However, exceptionally high-level aminoglycoside-resistance is achieved by the action of intrinsic and acquired 16S ribosomal RNA (rRNA) methyltransferase enzymes in aminoglycoside-producing and human pathogenic bacteria, respectively. These resistance determinants block drug binding by catalyzing the transfer of a methyl group from their cosubstrate S-adenosyl-l-methionine (SAM) to the base of a defined target RNA nucleotide within the ribosomal A-site. Here, we describe detailed structural and functional analyses of one of these enzymes, the kanamycin-resistance methyltransferase from Catenulisporales acidiphilia (‘CacKam’). CacKam has a SAM-binding core fold comprised of a seven-stranded β-sheet with a central topological switch point, characteristic of Class I methyltransferases.

To assess the relative contributions of these two interactions to the observed β6/7 linker structure, individual D21A and W203A substitutions were created for further functional and structural analyses. In contrast, substitution of the universally conserved W203 to alanine resulted in complete loss of resistance, consistent with previous analyses of equivalent substitutions in KamB and NpmA. In contrast, although CacKam-W203A also crystallized in space group P212121, the substitution results in a new unit cell with an altered packing arrangement and two molecules in the asymmetric unit. Changes in the CacKam-W203A structure are confined to the β6/7 linker, which is disordered in both chains. Additionally, D21 is no longer involved in crystal packing interactions made by either CacKam-W203A molecule. Thus, only direct disruption of the interaction of W203 with R43/ R73 through the W203A substitution is sufficient to induce changes in the β6/7 linker structure and the crystal lattice. Critically, in terms of β6/7 linker structure and dynamics in solution, the intensity of cleavage at R206 (bands c and d) is increased upon W203A, W203F or R43A/R73A substitution, consistent with increased flexibility in the absence of the R43/W203/R73 double cation–π interaction to stabilize the β6/7 linker conformation. In contrast, CacKam-W203A showed minimal methylation capacity, consistent with its inactivity in the MIC assay.

>[2x]MHHHHHHASGLVPRGSHMTRTTALKVLAGKKLTDLDPDEWAKAQASAERILVDVGTGDARTAYRQAIAHPEWLVVGVDPAWQRMTETAVRAARKPAKGGAPNLVLVSSAIETVPAALHGVADEVMVLMPWGKLLRGVVLGEADVLSGLRAVAKPGAPLEISIGTSIWREPIPLEIRDLPELTPETVVSTGLTDRLAALGWQVADVRLVPHTDLDTISSSAARRLGSGATETVLHLRAVAVDPRDPVGTQHPAAESAQDTPEEPQRDV>[4x]SNAQYEDGKQYTTLEKPVAGAPQVLEFFSFFCPHAYQFEEVLHISDNVKKKLPEGVKMTKYHVNFMGGDLGKDLTQAWAVAMALGVEDKVTVPLFEGVQKTQTIRSA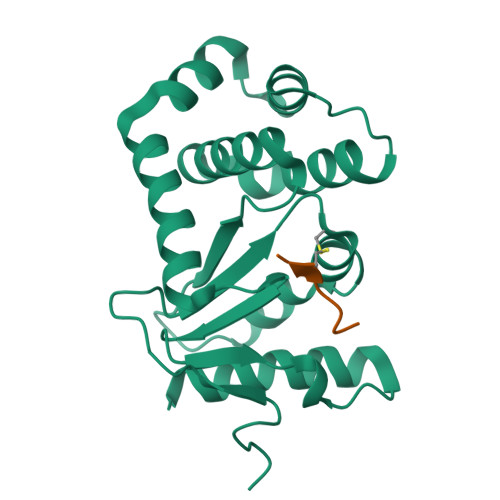SDIRDVFINAGIKGEEYDAAWNSFVVKSLVAQQEKAAADVQLRGVPAMFVNGKYQLNPQGMDTSNMDVFVQQYADTVKYLSEKK> MTQTTQSPALIASQSSWRCVQAHDREGWLALMADDVVIEDPIGKSVTNPDGSGIKGKEAVGAFFDTHIAANRLTVTCEETFPSSSPDEIAHILVLHSE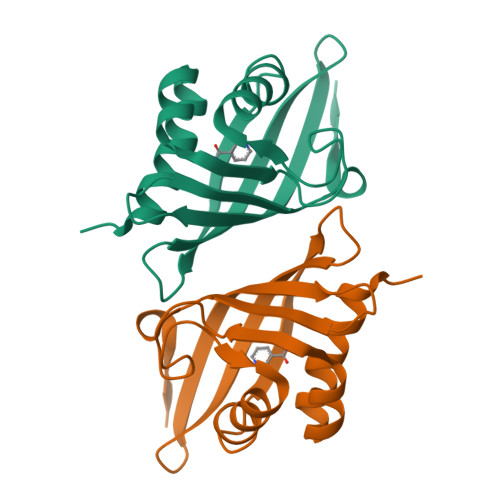FDGGFTSEVRGVFTYRVNKAGLITNMRGYWNLDMMTFGNQE>[4x]MQRNTYNKVGLYILSLAMLFVFIIILTAKIPFCFTSDCSFIGLKKLVLTNIVPIVCFVFFLFSIYFYNRLKNITKYNGQDSVKITSCQS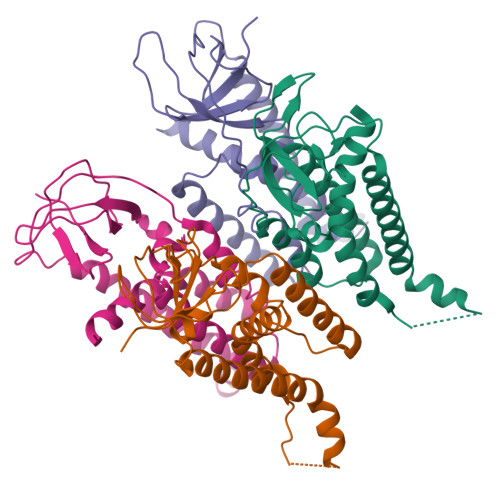ESYESLTFLATYIVPFMGFSFEDMQKNIAYLLLVVVIGIIFIKTDKYYANPTLALFGFKLYRVNILHPGSGETKNLIAISNDVLKVDDNVYYSFFDEFVFIARKKI Ctf4 forms a homotrimer that has the potential to connect the CMG helicase to one or two Pol α complexes, via the α-helical bundle at the carboxyl terminus of each Ctf4 protomer, which binds to a short conserved motif in the GINS component of CMG and the Pol1 catalytic subunit of Pol α (Simon et al., 2014). Here, we identify new Ctf4 partners in addition to Pol α and helicase, all of which contain a “Ctf4-interacting-peptide” or CIP-box. Crystallographic analysis classifies CIP-boxes into two related groups that target different sites on Ctf4. In addition to its role as a bridge between the CMG helicase and Pol α, our data indicate that Ctf4 functions as a key hub within the replisome, linking the helicase to a diverse set of partners.

The first of these was the multi-functional nuclease/helicase Dna2, which plays a role in the processing of Okazaki fragments during lagging strand synthesis, and in DNA-end resection for homologous recombination (Cejka, 2015, Kao and Bambara, 2003). Inspection of the amino acid sequence of Dna2 revealed a single peptide in its N-terminal region that closely resembled the Ctf4-interacting motif of Sld5 and Pol1. This sequence is located within the minimal fragment of Dna2 that interacted with Ctf4 in the two-hybrid screen, and associates directly with Ctf4 in vitro when fused to glutathione S-transferase (GST), in a manner that is dependent upon residues conserved with the equivalent motifs of Sld5 and Pol1. We then used non-dissociative (native) mass spectrometry and fluorescence anisotropy to show that an isolated peptide containing the Dna2 CIP-box was able to bind directly to Ctf4 in vitro. Encouraged by these findings, we soaked the Dna2 peptide into crystals of Ctf4 471–927, using the same approach that we described previously (Simon et al., 2014), and found that the Dna2 CIP-box sequence folded as a two-turn α helix that bound to the helical domain of Ctf4, in a very similar manner to the CIP-boxes of Sld5 and Pol1. These data indicate that budding yeast Dna2, Sld5, and Pol1 are archetypes of a set of CIP-box proteins that all share a common mode of interaction with Ctf4. The dna2-4A allele was viable, even in the absence of the Mec1 checkpoint kinase, indicating that displacement of Dna2 from Ctf4 does not produce significant defects in DNA synthesis. Interestingly, however, pulse field gel electrophoresis indicated that chromosome 12 was dramatically smaller in dna2-4A cells, whereas other chromosomes were not affected. This suggests that tethering of Dna2 to Ctf4 at replication forks is part of a replication-coupled mechanism to maintain the large array of rDNA repeats on chromosome 12.

>[3x]MGSSHHHHHHSQDPENLYFQGTGKFRYMPFSPAGTPFGFTDRRYLTMNEVGYVSTVKNSEQYSITVSFFDVGRFREYHFEDLFGYDLCFLNEKGTLFGQSKTGQIQYRPHDSIHSNWTKIIPLQAGERITSVAATPVRVIVGTSLGYFRSFNQFGVPFAVEKTSPIVALTAQNYRVFSVHYSQFHGLSYSLSELGTSSKRYYKRECPLPMSLPNINSDMKKDANLDYYNFNPMGIKSLFFSSYGDPCIFGSDNTLLLLSKWRSPEESKWLPILDSNMEIWKMSGGKETTDIHVWPLALAYDTLNCILVKGKHIWPEFPLPLPSEMEIRMPVFVKSKLLEENKAILNKKNEIGADTEAEEGEEDKEIQIPVSMAAEEEYLRSKVLSELLTDTLENDGEMYGNENEVLAALNGAYDKALLRLFASACSDQNVEKALSLAHELKQDRALTAAVKISERAELPSLVKKINNIREARYEQQLK;>[2x]SLRNIDDILDDIEGDLT> MNPNQKIITIGSVTLTIATICFLMQIAILVTTVTLHFKQYECNSPPNNQVMLCEPTIIERNITEIVYLTNTTIEKEICPKLAEYRNWSKPQCKITGFAPFSKDNSIRLSAGGDIWVTREPYVSCDPGKCYQFALGQGTTLNNRHSNDTVHDRTPYRTLLMNELGVPFHLGTKQVCIAWSSSSCHDGKAWLHVCVTGHDENATASFIYDGRLVDSIGSWSKNILRTQESECVCINGTCTVVMTDGSASERADTKILFIEEGKIVHISPLSGSAQHVEECSCYPRYPGVRCVCRDNWKGSNRPIVDINVKDYSIVSSYVCSGLVGDTPRKNDSSSSSYCRNPNNEKGSHGVKGWAFDDGNDVWMGRTISEELRSGYETFKVIGGWSKPNSKLQINRQVIVDRGNRSGYSGIFSVEGKSCINRCFYVELIRGRKQETEVWWTSNSIVVFC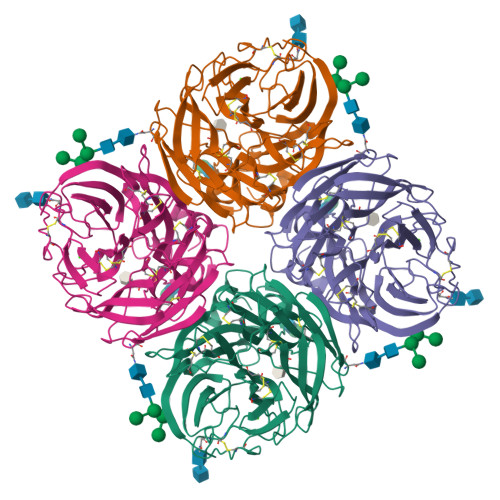GTSGTYGTGSWPDGGDINLMPI> MSLEKPKVERSEGKEKLEDYAYVLDFMPYGHPDDKRPIHRREPLAQ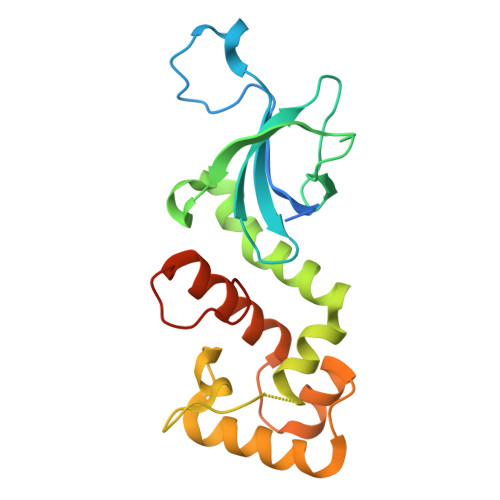VVGERNFTLLEVSIRKGKQPLVMDRVYIGKGERDVVYKIKRRLRYEDLTPAAKTELPYVIEHIIKQDEKKYVDFFNKADSITTRMHQLELLPGVGKKMMWAIIEERKKRPFESFEDIAQRVKGIQRPEKLIVSRIIYEIKNPQTKYKLFTAEGHHHHHH>[2x]GSHMNINKQSPIPIYYQIMEQLKTQIKNGELQPDMPLPSEREYAEQFGISRMTVRQALSNLVNEGLLYRLKGRGTFVSKPKMEQALQGLTSFTEDMKSRGMTPGSRLIDYQLIDSTEELAAILGCGHPSSIHKITRVRLANDIPMAIESSHIPFELAGELNESHFQSSIYDHIERYNSIPISRAKQELEPSAATTEEANILGIQKGAPVLLIKRTTYLQNGTAFEHAKSVYRGDRYTFVHYMDRLS

NagR, formerly termed YvoA, has been identified as a repressor protein from Bacillus subtilis that regulates genes involved in N-acetylglucosamine (GlcNAc) utilization. NagR acts as a negative transcriptional regulator, and binding of effector-free NagR to specific DNA operator sites blocks gene transcription. With more than 49000 deposited sequences, the GntR family of regulators (gluconate-operon repressor, Pfam family: PF00392) represents one of the largest groups of bacterial metabolite-responsive transcription factors. Their tertiary structure can be subdivided in almost all cases into two distinct domains: an N-terminal DNA-binding winged-helix-turn-helix (wHTH) domain and a C-terminal small-molecule effector-binding and oligomerization domain. In NagR and the entire GntR/HutC subfamily the C-terminal effector-binding domain adopts a so-called UTRA domain fold (Pfam family: PF07702) that is structurally homologous to the enzyme chorismate lyase.

The crystal structures of the complexes between NagR and GlcN-6-P as well as NagR and GlcNAc-6-P were solved at 2.1 and 2 Å, respectively. The two complexes crystallized isomorphously and their asymmetric unit contains one entire NagR homodimer. GlcN-6-P and GlcNAc-6-P are bound to NagR in an α-anomeric configuration. Each phosphate group is coordinated by the N-termini of helices αE1 (Thr90) and αE5 (Ser165, Ile166 and Tyr167) as well as by residues Arg133 and Arg135 presented by β-strand βE2. The sugar moieties are predominantly recognized via direct or water-mediated hydrogen bonds involving polar main and side chain atoms from residues Phe89, Glu145 and Tyr228 as well as via hydrophobic interactions with Ser88, Arg211, Glu222 and Ala224. The phosphorylated sugars stack against Tyr167 and form an additional CH/π interaction often observed in sugar–protein complexes. Whereas the acetyl component of GlcNAc-6-P is indirectly contacted by Ile209 and Ser226, the resulting additional space in the binding pocket in the case of GlcN-6-P is filled by a water molecule and an adjacent ethylene glycol (EDO) molecule from the cryoprotectant solution. However, upon binding of GlcN-6-P and GlcNAc-6-P, the DBDs are displaced even further by an additional 25 Å. The ligand-bound structures, however, now reveal an even more distinctive rearrangement of the DBDs and the formation of a novel beta-strand β* that interacts with the C-terminal strand βE7. This newly formed beta-strand β* appears to lock the DBD in the observed ‘upward’ positioning.>[2x]AIAMAELLTPKIVIIGAGPTGLGAAVRLTELGYKNWHLYECNDTPG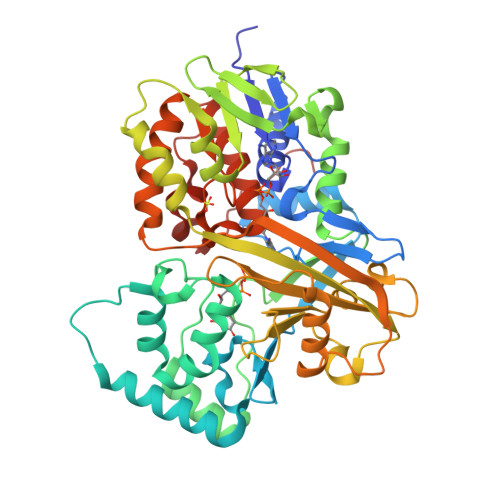GLSRSFLDENGFTWDLGGHVIFSHYQYFDDVMDWAVQGWNVLQRESWVWVRGRWVPYPFQNNIHRLPEQDRKRCLDELVRSHARTYTEPPNNFEESFTRQFGEGIADIFMRPYNFKVWAVPPCLMSTEWVEERVAPVDLERIRRNIQENRDDLGWGPNATFRFPQRGGTGIIYQAIKEKLPSEKLTFNSGFQAIAIDADAKTITFSNGEVVSYDYLISTVPFDNLLRMTKGTGFKGYDEWPAIADKMVYSSTNVIGIGVKGTPPPHLKTACWLYFPEDTSPFYRATVFSNYSKYNVPEGHWSLMLEVSESKYKPVNHSTLIEDCIVGCLASNLLLPEDLLVSKWHYRIEKGYPTPFIGRNNLLEKAQPELMSRCIYSRGRFGAWRYEVGNQDHSFMQGVEAIDHVLGLATEETTVANPGRVNGTRATTHFGLLQKDMV>[2x]CGIWALFGSDDCLSVQCLSAMKIAHRGPDAFRFENVNGYTNCCFGFHRLAVVDPLFGMQPIRVKKYPYLWLCYNGEIYNHKKMQQHFEFEYQTKVDGEIILHLYDKGGIEQTICMLDGVFAFVLLDTANKKVFLGRDTYGVRPLFKAMTEDGFLAVCSEAKGLVTLKHSATPFLKVEPFLPGHYEVLDLKPNGKVASVEMVKYHHCRDVPLHALYDNVEKLFPGFEIETVKNNLRILFNNAVKKRLMTDRRIGCLLSGGLDSSLVAATLLKQLKEAQVQYPLQTFAIGMEDSPDLLAARKVADHIGSEHYEVLFNSEEGIQALDEV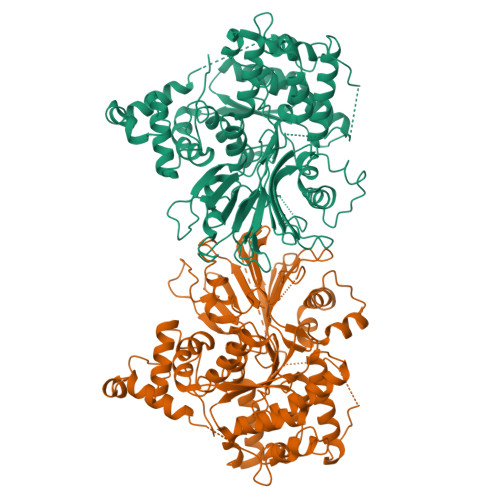IFSLETYDITTVRASVGMYLISKYIRKNTDSVVIFSGEGSDELTQGYIYFHKAPSPEKAEEESERLLRELYLFDVLRADRTTAAHGLELRVPFLDHRFSSYYLSLPPEMRIPKNGIEKHLLRETFEDSNLIPKEILWRPKEAFSDGITSVKNSWFKILQEYVEHQVDDAMMANAAQKFPFNTPKTKEGYYYRQVFERHYPGRADWLSHYWMPKWINATDPSARTLTHYKSAVKA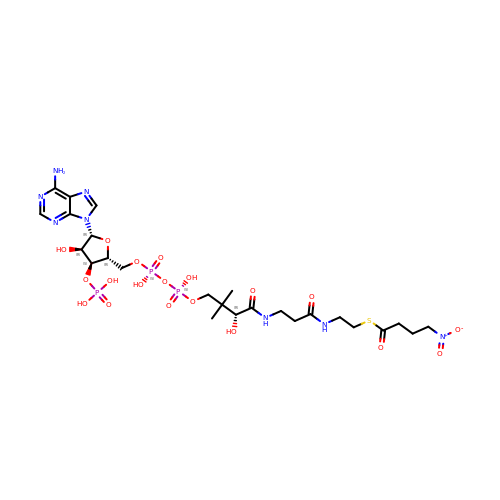S-4-NITROBUTYRYL-COA | C25 H41 N8 O19 P3 S | PXNIOQHGCSEKCC-CITAKDKDSA-N>[6x]GIDFPTMLKIKLEKTTFENAKAECSLVFIINKDFSHAWVKNKELLETFKYEGEGVFLDQENKILYAGVKEDDVHLLRESACLAVRTLKKLAFKSVKVGVYTCGAHSKDNALLENLKALFLGLKLGLYEYDTFKSNKKESVLKEAIVALELHKPCEKTCANSLEKSAKEALKYAEIMTESLNIVKDLVNTPPMIGTPVYMAEVAQKVAKENHLEIHVHDEKFLEEKKMNAFLAVNKASLSVNPPR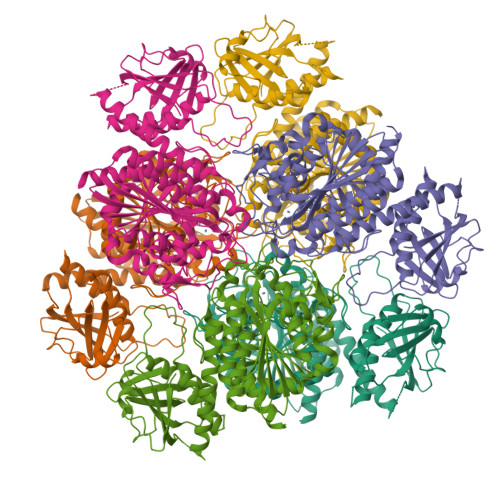LIHLVYKPKKAKKKIALVGKGLTYDCGGLSLKPADYMVTMKADKGGGSAVIGLLNALAKLGVEAEVHGIIGATENMIGPAAYKPDDILISKEGKSIEVRNTDAEGRLVLADCLSYAQDLNPDVIVDFATLTGACVVGLGEFTSAIMGHNEELKNLFETSGLESGELLAKLPFNRHLKKLIESKIADVCNISSSRYGGAITAGLFLNEFIRDEFKDKWLHIDIAGPAYVEKEWDVNSFGASGAGVRACTAFVEELLKKA EICOSA-8,11,14-TRIENOIC ACID | C20 H34 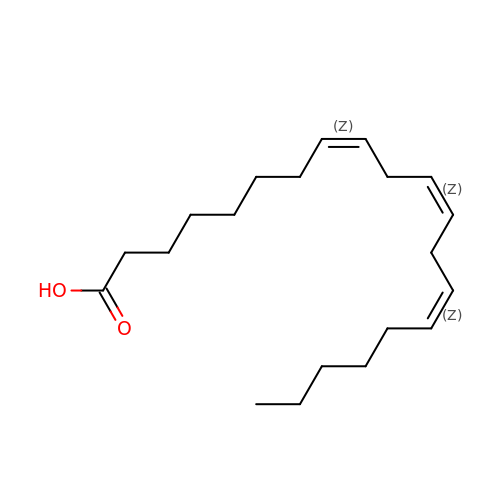O2 | HOBAELRKJCKHQD-QNEBEIHSSA-N>[6x]MHHHHHHMFSRFSNVVSEIEKKYVDKISISEIMTKAIEGLLSNLDAHSAYLNEKKFKEFQAQTEGEFGGLGITVGMRDGVLTVIAPLEGTPAYKAGVKSGDNILKINNESTLSMSIDDAINLMRGKPKTPIQITIVRKNEPKPLVFNIIRDIIKLPSVYVKKIKETPYLYVRVSGFDKNVTKSVLEGLKANPKAKGIVLDLRGNPGGLLNQAVGLSN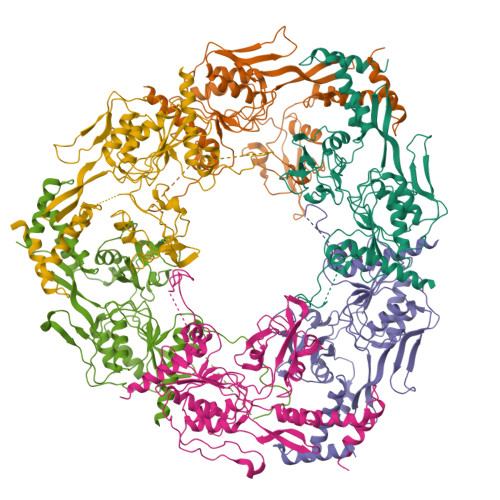LFIKEGVLVSQKGKNKEESLEYKANGRAPYTNLPIAVLVNGGSASASEIVAGALQDHKRAVIIGEKTFGKGSVQMLLPVNKDEAIKITTARYYLPSGRTIQAKGITPDIVIYPGKVPENENKFSLKEADLKHHLEQELKKLDDKTPNSKEADKDKKNEEEKEVTPKMINDDIQLKTAIDSLKTWSIVDEKMDEKAPKKK>[3x]GAMGSLIRKKAAGLESAATIRTKVFVWGLNDKDQLGGLKGSKIKVPSFSETLSALNVVQVAGGSKSLFAVTVEGKVYACGEATNGRLGLGISSGTVPIPRQITALSSYVVKKVAVHSGGRHATALTVDGKVFSWGEGDDGKLGHFSRMNCDKPRLIEALKTKRIRDIACGSSHSAALTSSGELYTWGLGEYGRLGHGDNTTQLKPKMVKVLLGHRVIQV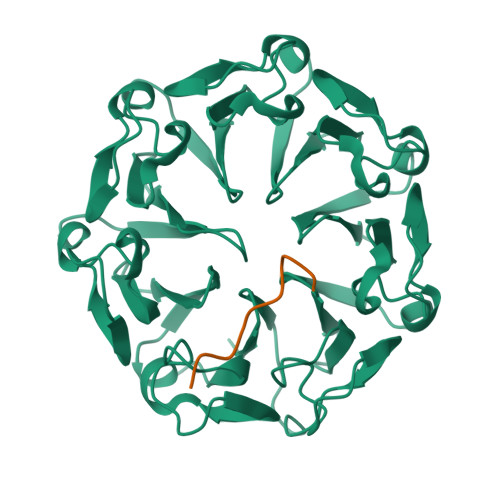ACGSRDAQTLALTDEGLVFSWGDGDFGKLGRGGSEGCNIPQNIERLNGQGVCQIECGAQFSLALTKSGVVWTWGKGDYFRLGHGSDVHVRKPQVVEGLRGKKIVHVAVGALHCLAVTDSGQVYAWGDNDHGQQGNGTTTVNRKPTLVQGLEGQKITRVACGSSHSVAWTTVDVATPSVHEPVLFQT;>EDDDDKDQDESDSDT[3x]> SSGHMRSTVFSDEEFSNILNDFPALKRNINGKRLVYLDNAASTLKCKSVIEKMTDFYLYHYSNIHRAVHTLASEATVAYEQAREKVANFLNASSEEIIFTSGTTMGINFLVNSLAKSGILKTEDTVLISQVEHHANLVPWVRLSKFYGFKVAYITADEKGVITNESILKTKESIPNPKVVSITGQSNVTGQEMPIELIRETFKNATLIVDGAQLVPHKKVDVKKLDVDFLVFSGHKILGPTGIGVLYGKKALLEQLEPFLYGGEMIDKVTFEDVTFNVLPYRFEAGTQHITGAVGLGYTIDYLESIGFEKVEKHVEELSNYLLEKMMELDFVEVYGPIDSSHKSLVSFNVKGVHPHDVSHILDENFGVATRSG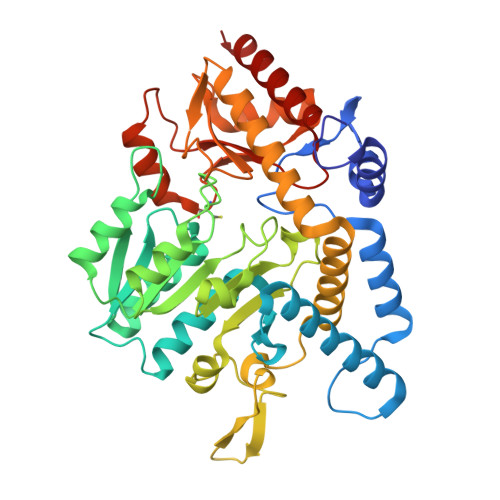HHCAQPLMGVLAKGSKIDFPNSTVRASVYLYNTKEDIDVLIEGLKYIRRWFE> ATFEIVNRCSYTVWAAASKGDAALDAGGRQLNSGESWTINVEPGTNGGKIWARTDCYFDDSGSGICKTGDCGGLLRCARFGRPPTTLAEFSLNQYGKDYIDISNIKGFNVPMDFSPTTRGCRGVRCAADIVGQCPAKLKAPGGGCNDACTVFQTSEYCCTTGKCGPTEYSRFFKRLCPDAFSYVLDKPTTVTCPGSSNY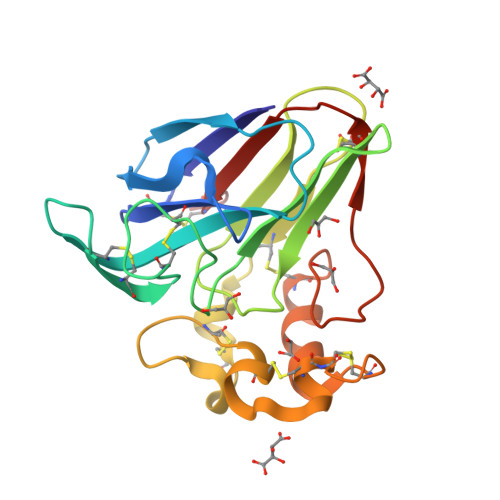RVTFCPTA> TSTDWK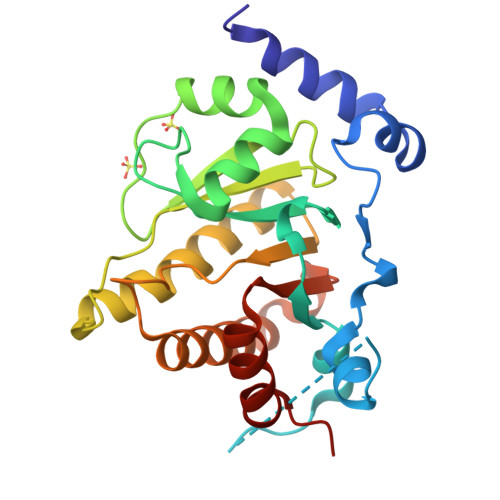EAKSFLKGLSDKQREEHYFCKDFVRLKKIPTWKEMAKGVAVKVEEPRYKKDKQLNEKISLLRSDITKLEVDAIVNAANSSLLGGGGVDGCIHRAAGPLLTDECRTLQSCKTGKAKITGGYRLPAKYVIHTVGPIAYGEPSASQAAELRSCYLSSLDLLLEHRLRSVAFPCISTGVFGYPCEAAAEIVLATLREWLEQHKDKVDRLIICVFLEKDEDIYRSRLPHYFPVA>[8x]RKFFVGGNWKMNGRKQSLGELIGTLNAAKVPADTEVVCAPPTAYIDFARQKLDPKIAVAAQNCYKVTNGAFTGEI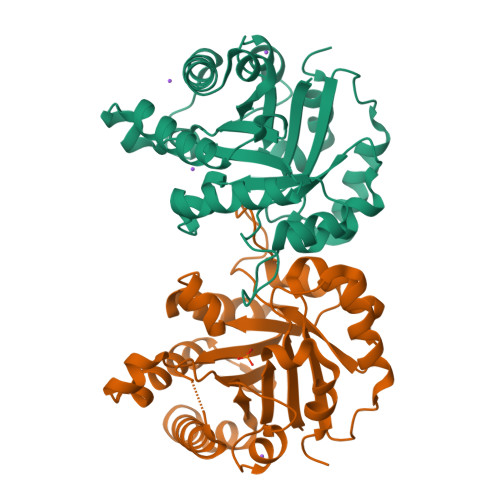SPGMIKDCGATWVVLGHSERRHVFGESDELIGQKVAHALAEGLGVIACIGEKLDEREAGITEKVVFEQTKVIADNVKDWSKVVLAYEPVWAIGTGKTATPQQAQEVHEKLAGWLKSNVSDAVAQSTRIIYGGSVTGATCKELASQPDVDGFLVGGASLKPEFVDIINAKQ> PNGQTKPLPALKLALEYIVPCMNKHGICVVDDFLGKETGQQIGDEVRALHDTGKFTDGQLVSQKSDSSKDIRGDKITWIEGKEPGCETIGLLMSSMDDLIRHCNGKLGSYKINGRTKAMVACYPGNGTGYVRHVDNPNGDGRCVTCIYYLNKDWDAKVSGGILRIFPEGKAQFADIEPKFDRLLFFWSDRRNPHEVQPAYATRYAITVWYFDADERAAAK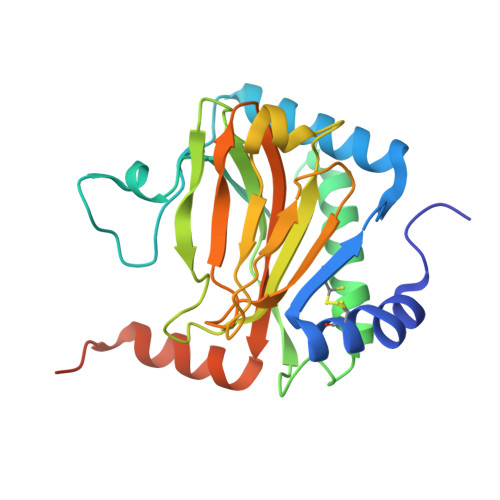VKYLTGEKGVRVELNKPSDSVGKDVF6-iodanyl-1~{H}-indole-2-carboxylic acid | C9 H6 I N O2 | 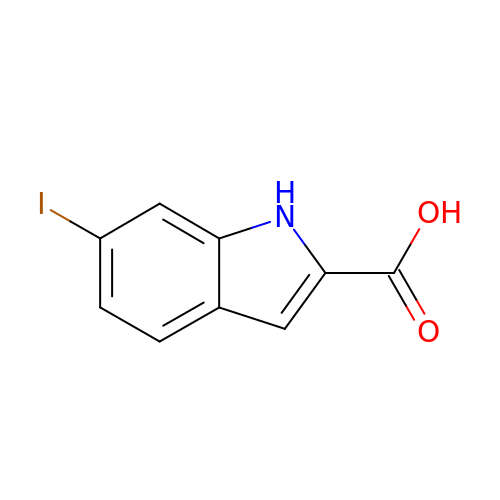LLSYKFHQMUBJCF-UHFFFAOYSA-N> MVPPTINTGKNITTERAVLTLNGLQIKLHKVVGESRDDIVAKMKDLAMDDHKFPRLPGPNPVSIERKDFEKLKQNKYVVSEKTDGIRFMMFFTRVFGFKVCTIIDRAMTVYLLPFKNIPRVLFQGSIFDGELCVDIVEKKFAFVLFDAVVVSGVT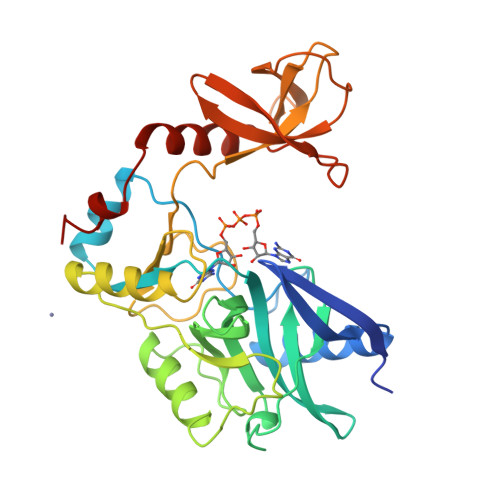VSQMDLASRFFAMKRSLKEFKNVPEDPAILRYKEWIPLEHPTIIKDHLKKANAIYHTDGLIIMSVDEPVIYGRNFNLFKLKPGTHHTIDFIIMSEDGTIGIFDPNLRKNVPVGKLDGYYNKGSIVECGFADGTWKYIQGRSDKNQANDRLTYEKTLLNIEENITIDELLDLFKWE> CFTARMSPP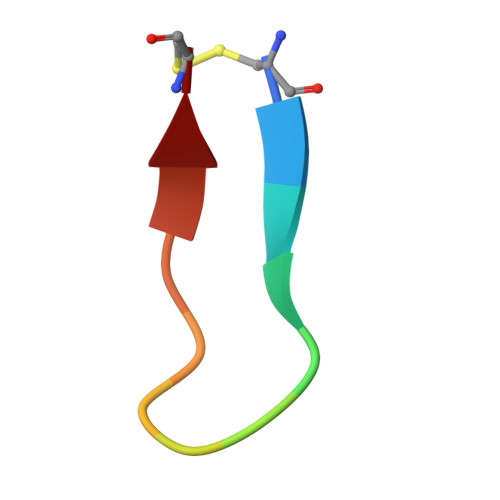QQIC>MVKEFNTQTELSVRLEALWAVLSKDFITVVPKVLPHIVKDVQLIEGDGGVGTILIFNFLPEVSPSYQREEITEFDESSHEIGLQVIEGGYLSQGLSYYKTTFKLSEIEEDKTLVNVKISYDH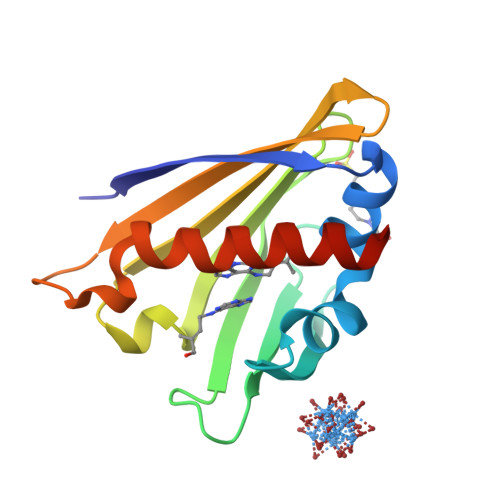DSDIEEKVTPTKTSQSTLMYLRRLERYLSNGSA[4x]>GSHMKNSVSVDLPGSMKVLVSKSSNADGKYDLIATVDALELSGTSDKNNGSGVLEGVKADASKVKLTISDDLGQTTLEVFKSDGSTLVSKKVTSKDKSSTYEKFNEKGELSEKYITRADKSSTYEKFNEKGELSEKYITRADKSSTYE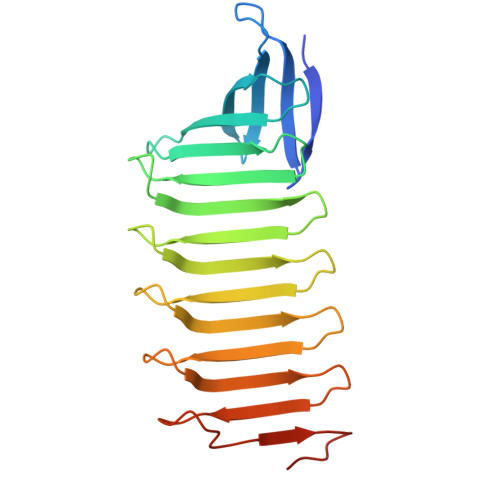KFNEKGELSEKYITRADKSSTYEKFNEKGEVSEKYITRADGTRLEYTGIK[4x]> QEITVDEFSNIRENPVTPANPEPSAPVIDPTAYI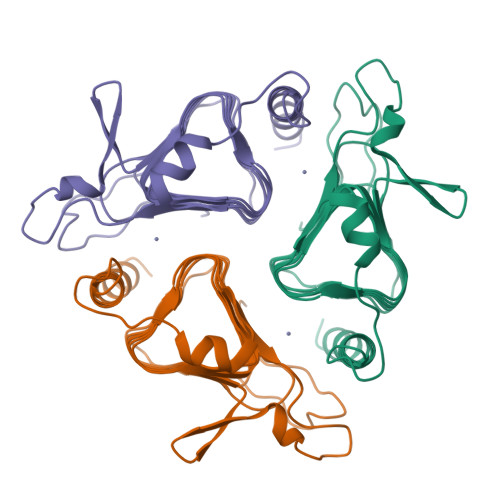DPQASVIGEVTIGANVMVSPMASIRSDEGMPIFVGDRSNVQDGVVLHALETINEEGEPIEDNIVEVDGKEYAVYIGNNVSLAHQSQVHGPAAVGDDTFIGMQAFVFKSKVGNNCVLEPRSAAIGVTIPDGRYIPAGMVVTSQAEADKLPEVTDDYAYSHTNEAVVYVNVHLAEGYKETS5'-O-{[(2,3-dihydroxyphenyl)carbonyl]sulfamoyl}adenosine | C17 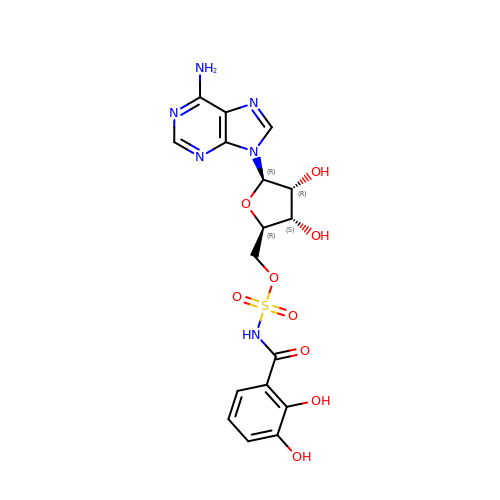H18 N6 O9 S | DDOFAAYVEMVKLG-DMEFTLKTSA-N> TIGSEFKPHISALNAPSLAQRYKDYFYIGAAVE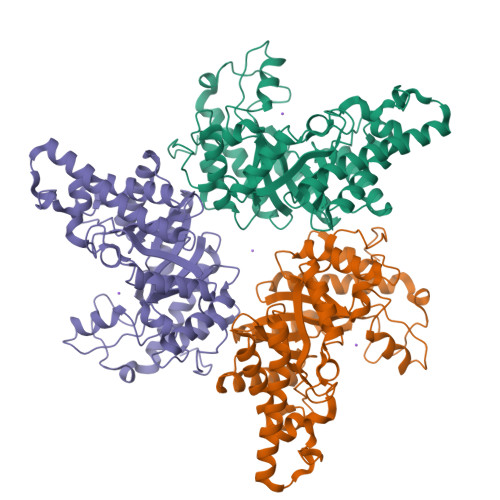PYQTTKEKDAKMLQRHFNMIVAENAMKPAALEPTEGNFQWADADRIVQFAKENGMELRFHTLVWHNQTPDWFFLDREGKPMVEETDPQKREENRELLLQRLENHIRAVVLRYKDDIKNWDVVNEVVEPNDPGGMRNSPWYQITGTEYIEVAFRAAREAGGEDIKLYMNDYNTEQEPKREYIYRLIKKLLEKGVPIDGVGHQAHVTIDRPPVDEIKKTIQRFADLGLDNQITELDVSLYGWPPRPAYPTYDAIPEERFQAQADRYRQLFELFEELKDHISAVTFWGIADNHTWLDDRAREYNDGVGKDAPFVFDPNYRVKPAYWAIINHK>[8x]MSEKKNIYPN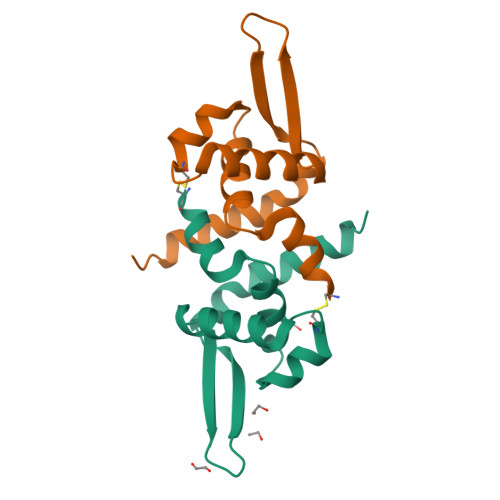KEGCPVEFTLDVIGGKWKGILFYHMIDGKKRFNEFRRICPSITQRMLTLQLRELEADGIVHREVYHQVPPKVEYSLTEFGRTLEPIVLQMKEWGESNRDVLESYRSNGLVKDQQKHHHHHH> MTLAEPTKDTPPVEMVSLTIDDHEISVPKGTLLIRAAELMGIQIPRFCDHPLLDPVGACRQCLVEVEGQRKPMASCTTTVMPDMVVRTQFTSEAADKAQRGVMELLLINHPLDCPICDKGGECPLQNQAMSNGRPETRFEDVKRTFPKPISISSQVLLDRERCVLCARCTRFSSQIAGDPFIDLMERGALQQVGIGQDKPFQSYFSGN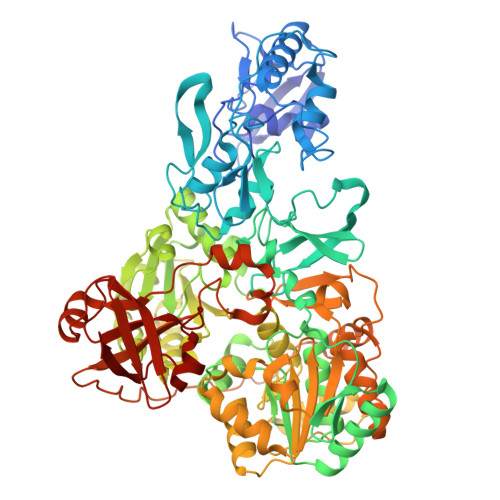TVQICPVGALTGTAYRFRARPFDLVSSPSVCEHCASGCAQRTDHRRGKVLRRLAGDEPEVNEEWNCDKGRWAFTYATVGDRITTPMLRDGGVLRPASWSEALTVAAAGLLTAAGSTGVLVGGRCTVEDAYAYAKFARMVLNTNDVDFRARPHSAEEAEFLAAHVAGQTMGLRYAELENAPTVLLAGFEPEEESPIVFLRLRKGVRKNGVQVVAVAPWASRGLTKLAGTVVPTVPGDEPAALDGMHDDDRLRRPGAVILVGERLATSPGALSAAVRLAAATGARLAWIPRRAGERGAIEAGALPNLLPGGRPVDDADARAEVARAWYISALPEAPGRDTAAILSTAASGHLAALLVGGVELGDLPDPELAVAAVRTTPFVVSLELRESAVTELADVVFPVAPVVEKAGSFLNWEGRPRPFAPSLKTNAIPDLRVLHYLADEIGVDLALPTAEAADAELAQLGTWGGARPPAPTAPPTARPEAGSGQAVLASWRMLLDAGRLQDGEPHLAGTAVRPVARMSAATAAGIGASDGAPVTVSTERGAVTLPLAVTDMPDGVVWLPMNSPGSAVHQRLGVTAGAVVSIGAGA>NAMSVVIERIPKEAIPKSLLL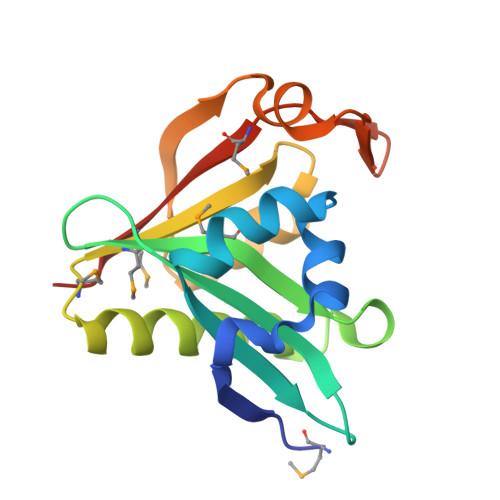LADPSERQIATYVQRGLTYVAKQGGSVIGVYVLLETRPKTMEIMNIAVAEHLQGKGIGKKLLRHAVETAKGYGMSKLEVGTGNSSVSQLALYQKCGFRIFSIDFDYFSKHYEEEIIENGIVCRDMIRLAMELNKNV[4x]> MIHHVELTQSVLQY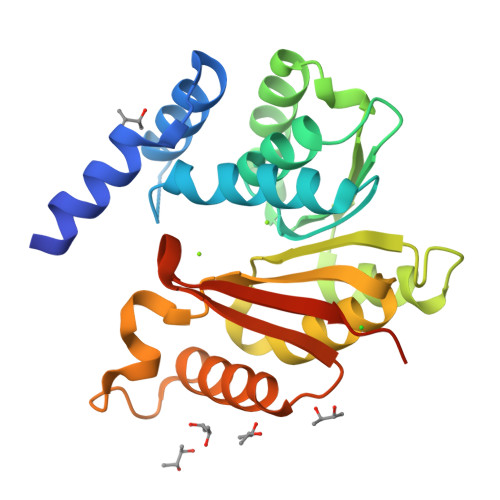IRDSSVRDNDILRDLREETSKLPLRTMQIPPEQGQLLSLLVRLIGARKTLEVGVFTGYSTLCTALALPADGRVIACDLSEEWVSIARRYWQRAGVADRIEVRLGDAHHSLEALVGSEHRGTFDLAFIDADKESYDFYYEHALRLVRPGGLIILDNTLWSGKVADPSVVGDPETDSLRRINAKLLTDERVDLSMLPIADGLTLARKRKLAAALEHHHHHH Cyclic nucleotide binding domains (CNB) confer allosteric regulation by cAMP or cGMP to many signaling proteins, including PKA and PKG. PKA of phylogenetically distant Trypanosoma is the first exception as it is cyclic nucleotide-independent and responsive to nucleoside analogues. Here, we show that natural nucleosides inosine, guanosine and adenosine are nanomolar affinity CNB ligands and activators of PKA orthologs of the important tropical pathogens Trypanosoma brucei, Trypanosoma cruzi, and Leishmania. Substitution of two to three amino acids in the binding sites is sufficient for conversion of CNB domains from nucleoside to cyclic nucleotide specificity.

To evaluate the binding mode, we solved the crystal structures of T. cruzi PKAR(200-503) and T. brucei PKAR(199-499) bound to inosine at 1.4 Å and 2.1 Å resolution, respectively. The structures of TbPKAR and TcPKAR show high overall similarity. (b) T. brucei PKAR(199-499) displayed as in A, Residues G308, E309, E311, and A320 are part of RBC-A while G432, E433, and E435 belong to RBC-B. Capping residues (Y370 and Y482) are marked with an asterisk. The glutamates in kinetoplastid RBCs interacts with the 3’ and 5’ OH groups of ribose. Moreover, the arginines 209/333PKARIα and the glutamates 311/435TbPKAR occupy the same spatial position in the structures. A superposition of the mammalian and T. brucei structures shows a clash between the phosphate group of cAMP and the negatively charged side chain of E311/435TbPKAR. The high-resolution crystal structures of T. brucei PKAR and T. cruzi PKAR thus provides a molecular rationale for absence of binding and activation by cAMP. In the ligand-bound structures of TbPKAR and TcPKAR, this helix docks to theβ-barrel of the B-site, covers the binding pocket and shields the ligand from solvent. Y484 interacts with the backbone of V443 and R413 while Y485 forms two hydrogen bonds to the side chains of N438 and H440. The beta factor representation of TbPKAR suggests that proline 480 functions as a hinge between αC and αD, as the average displacement of P480 is higher than that of the other residues around it, likely correlating with higher mobility.

>[2x]GRKRRTTVRGEGIDPEKAKSYVAPYFEKSEDETALILKLLTYNVLFSFLDSRDLMTVAGAMWRVEFKQDDCIMEAGQTTCDKLYIIQDGKADIIKEGQKVYLKVEGTAVGELELMYQTPTVATVKVCTPELIAWALDRDTYRHLVMGSAIRRRETYIQFLTNIPFLSGLDNYEKLQLADALSSDEFEPGDYIIRYGEEGEWLYIILEGSVDVVGRDDDGNEKHVWEFGKGDHVGELEFLNNHANVADVVAKTHVVTAKLNRRHFEMCLGPVIDVLKRTSQQPNYEYYQSKLKTTLRAEGRK> MSSTVISRKRRNSTVTEPDSSGETRKQKKSRSDEKSSSSKDGDPQLEFKVLQGYRDLESEMHKGRAQVTRTGDIGVAMDNLNAVDSLFNKVIGIKNNGLFAHDARAMVSISELAQISVRNLKFDDSRSMVNLENIVNSLKRYMLKEHFKLNNIAENRNDLTL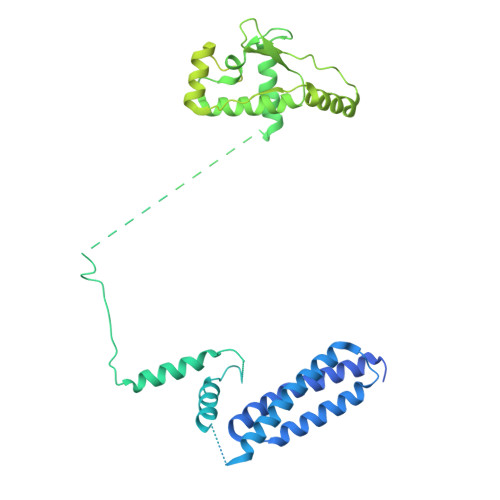AADEQSAADQQEESDGDIDRTPDDNHTDKATSSFKATSMRHSYLQQFSHYNEFSQFNWFRIGALYNTISKNAPITDHLMGPLSIEKKPRVLTQRRRNNDQVGEKITAEKITQHSLNSTQQETTPEQVKKCFKKLSKKLGPEGSINLFKFIIDPNSFSRSIENLFYTSFLIKEGKLLMEHDEEGLPTIKIKQSISHTDSRSKEIERQRRRAAHQNHIIFQMDMPTWRKLIKKYNITSPFLDGSSGMAEIGTGFPFDPHYVEVLGERMHYVDVGPRDGTPVLFLHGNPTSSYVWRNIIPHVAPTHRCIAPDLIGMGKSDKPDLGYFFDDHVRFMDAFIEALGLEEVVLVIHDWGSALGFHWAKRNPERVKGIAFMEFIRPIPTWDEWPEFARETFQAFRTTDVGRKLIIDQNVFIEGTLPMGVVRPLTEVEMDHYREPFLNPVDREPLWRFPNELPIAGEPANIVALVEEYMDWLHQSPVPKLLFWGTPGVLIPPAEAARLAKSLPNCKAVDIGPGLNLLQEDNPDLIGSEIARWLSTLEISGGSEQKLISEEDL5'-{[(3S)-3-amino-3-carboxypropyl]({1-[(thiophen-2-yl)methyl]azetidin-3-yl}methyl)amino}-5'-deoxyadenosine 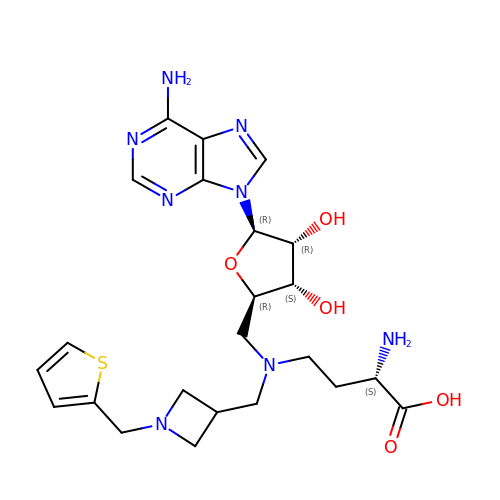| C23 H32 N8 O5 S | KJOQVBZBXKPYJX-XVZIYINBSA-N> SNAMAFIQTDTFTLRGYECDAFGRMSIPALMNLMQESANRNAIDYGIGIADLAQKGVGWMLMRFCLRIHQYPRYGDTIQLMTYPTTVDKYFIHRDFRVLATDGTLLADARSTWLVFSMEKRSMVPLPDFIRQLSPPANVDPLPALPLKPDFQTASFATAASKSVQVGWLNIDQNQHVNNVAYVQWLLEGVDSEIVQT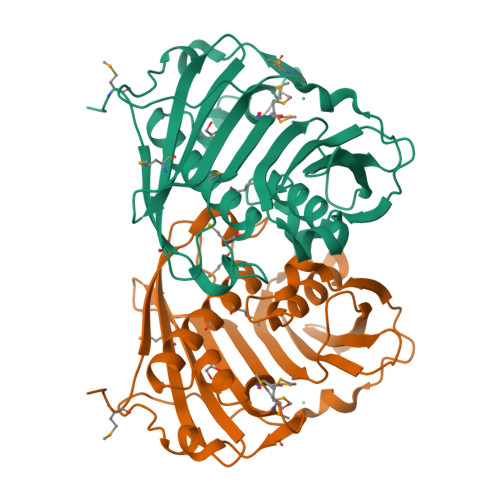REIAEIDLVYRTESHWHDWLSVQSVTETDNSVLHRISQTESGKDVLLARSRWR> SRNFIIPKKEIHTVPDMGKWKRSQAYADYIGFILTLNEGVKGKKLTFEYRVSEAIEKLVALLNTLDRWIDETPPVDQPSRFGNKAYRTWYAKLDEEAENLVATVVPTHLAAAVPEVAVYLKESVGNSTRIDYGTGHEAAFAAFLCCLCKIGVLRVDDQIAIVFKVFNRYLEVMRKLQKTYRMEPAGSQGVWGLDDFQFLPFIWGSSQLIDHPYLEPRHFVDEKAVNENHKDYMFLECILFITEMKTGPFAEHSNQLWNISAVPSWSKVNQGLIRMYKAE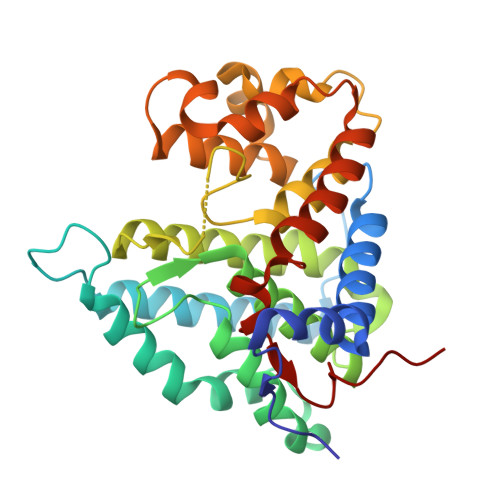CLEKFPVIQHFKFGSLLPIHPVTSG> PVTINNFNYNDPIDNNNIIMMEPPFARGTGRYYKAFKITDRIWIIPERYTFGYKPEDFNKSSGIFNRDVCEYYDPDYLNTNDKKNIFLQTMIKLFNRIKSKPLGEKLLEMIINGIPYLGDRRVPLEEFNTNIASVTVNKLISNPGEVERKKGIFANLIIFGPGPVLNENETIDIGIQNHFASREGFGGIMQMKFCPEYVSVFNNVQENKGASIFNRRGYFSDPALILMHELIHVLHGLYGIKVDDLPIVPNEKKFFMQSTDAI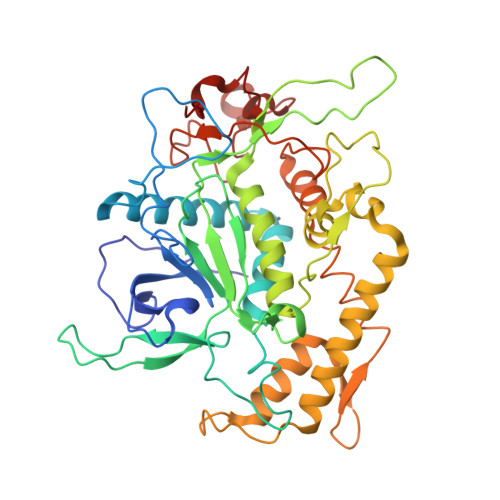QAEELYTFGGQDPSIITPSTDKSIYDKVLQNFRGIVDRLNKVLVCISDPNININIYKNKFKDKYKFVEDSEGKYSIDVESFDKLYKSLMFGFTETNIAENYKIKTRASYFSDSLPPVKIKNLLDNEIYTIEEGFNISDKDMEKEYRGQNKAINKQAYEEIS>[4x]SPLAAYEVDDSTGYLTSDVGGPIQDQTSLKAGIRGPTLLEDFMFRQKIQHFDHERVPERAVHARGAGAHGTFTSYADWSNITAASFLNATGKQTPVFVRFSTVAGSRGSADTARDVHGFATRFYTDEGNFDIVGNNIPVFFIQDAIQFPDLIHSVKPRPDNEIPQAATAHDSAWDFFSQQPSTMHTLFWAMSGHGIPRSYRHMDGFGCHTFRFVKDDGSSKLIKWHFKSRQGKASLVWEEAQVLSGKNADFHRQDLWDAIESGNGPEWDVCVQIVDESQAQAFGFDLLDPTKIIPEEYAPLTKLGLLKLDRNPTNYFAETEQVMFQPGHIVRGIDFTEDPLLQGRLFSYLDTQLNRNGGPNFEQLPINMPRVPIHNNNRDGAGQMFIHRNKYPYTPNTLNSGYPRQANQNAGRGFFTAPGRTASGALVREVSPTFNDHWSQPRLFFNSLTPVEQQFLVNAMRFEISLVKSEEVKKNVL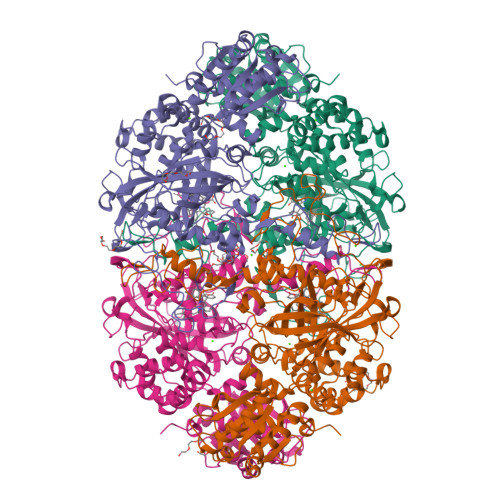TQLNRVSHDVAVRVAAAIGLGAPDADDTYYHNNKTAGVSIVGSGPLPTIKTLRVGILATTSESSALDQAAQLRTRLEKDGLVVTVVAETLREGVDQTYSTADATGFDGVVVVDGAAALFASTASSPLFPTGRPLQIFVDAYRWGKPVGVCGGKSSEVLDAADVPEDGDGVYSEESVDMFVEEFEKGLATFRFTDRFALDS> MTKTITVAHIQYDFKAVLEENDENDDEFYINVDKNLNEIKEHKIVVLGNSRGVDAGKGNTFEKVGSHLYKARLDGHDFLFNTIIRDGSKMLKRADYTAVDTAKL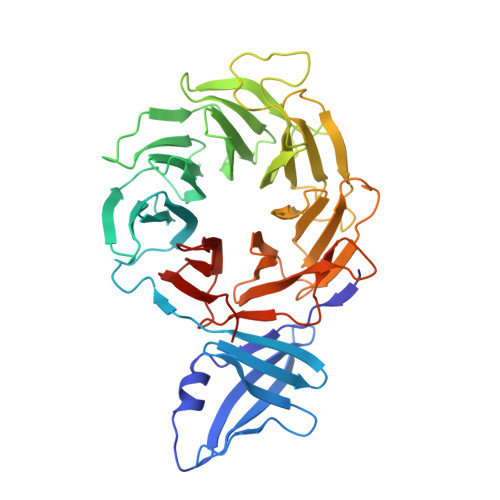QMRRFILGTTEGDIKVLDSNFNLQREIDQAHVSEITKLKFFPSGEALISSSQDMQLKIWSVKDGSNPRTLIGHRATVTDIAIIDRGRNVLSASLDGTIRLWECGTGTTIHTFNRKENPHDGVNSIALFVGTDRQLHEISTSKKNNLEFGTYGKYVIAGHVSGVITVHNVFSKEQTIQLPSKFTCSCNSLTVDGNNANYIYAGYENGMLAQWDLRSPECPVGEFLINEGTPINNVYFAAGALFVSSGFDTSIKLDIISDPESERPAIEFETPTFLVSNDDEVSQFCYVSDDESNGEVLEVGKNNFCALYNLSNP>[2x]MEKDGLCRADQQYECVAEIGEGAYGKVFKARDLKNGGRFVALKRVRVQTGEEG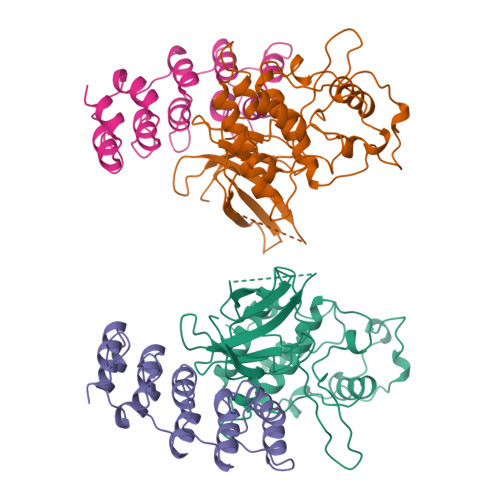MPLSTIREVAVLRHLETFEHPNVVRLFDVCTVSRTDRETKLTLVFEHVDQDLTTYLDKVPEPGVPTETIKDMMFQLLRGLDFLHSHRVVHRDLKPQNILVTSSGQIKLADFGLARIYSFQMALTSVVVTLWYRAPEVLLQSSYATPVDLWSVGCIFAEMFRRKPLFRGSSDVDQLGKILDVIGLPGEEDWPRDVALPRQAFHSKSAQPIEKFVTDIDELGKDLLLKCLTFNPAKRISAYSALSHPYFQDLERCKENLDSHLPPSQNTSELNTA;>MLLEEVRAGDRLSGAAARGDVQEVRRLLHRELVHPDALNRFGKTALQVMMFGSTAIALELLKQGASPNVQDTSGTSPVHDAARTGFLDTLKVLVEHGADVNVPDGTGALPIHLAVQEGHTAVVSFLAAESDLHRRDARGLTPLELALQRGAQDLVDILQGHMVAPL[2x]>GSMNLIPTVIETTNRGERAYDIYSRLLKDRIIMLGSQIDDNVANSIVSQLLFLQAQDSEKDIYLYINSPGGSVTAGFAIYDTIQHIKPDVQTICIGMAASMGSFLLAAGAKGKRFALPNAEVMIHQPLGGAQGQATEIEIAANHILKTRE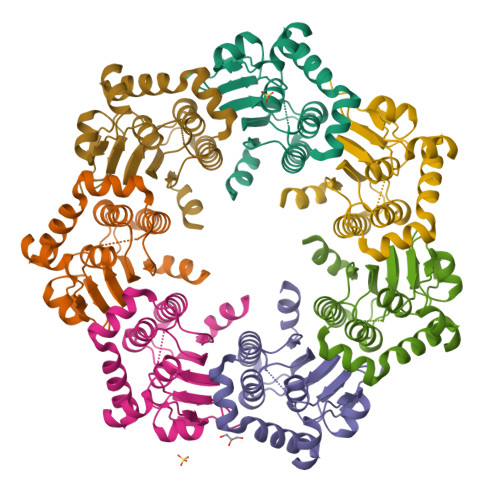KLNRILSERTGQSIEKIQKDTDRDNFLTAEEAKEYGLIDEVMVPETK[7x]>[2x]GSAMGSSTSTSRATYMDRFNIPKNHVDLIWDKDGTKSHTRGNTTYRWTERKSNVGVYVGYSEMYDSSAQAYCQSSSAKIDTKTTVGAPYMAAGACPNYGKVIAFTKRDGSRSDMTRWKNEIHANVMPHSTTSCASRADPGAAEVAKSIEGFAMYAGYLTHCPYNVNVYRQDMVTDKEFDSTVCNFVTESNPLRFLDTTQRQSTQPYTEYAFHGKGGHKGYDYKGQTSHVGCPPYNPPHVTKGMKDSSWITGPFECSILSRCTTHCWPYKSGGNCFRSLPAMFDMSTGECRLLGYHTQDFRSSTCAELTTDDTNAFYCVRPMKTAASSNMVYVTSHTRPDHETKCPP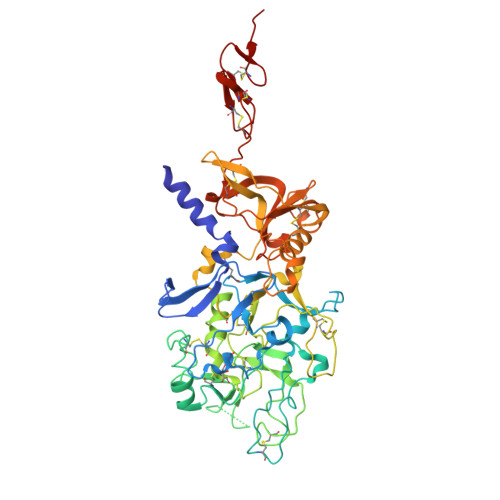REPLKNVRWGVVSKGKYCKPMNARASLSNATAEQCGQRLFMLSSADGSSLSSQVRGYHWATFVATDCNMGESCAATARGKCFFYSTVPECLIHSPTTMAFTSLSAVDPSIAIDPDSIAVLPEDKCVSVDCGAHGTCDVATGKCVCEPGFTGERCDAAALVPR> SAGSKSCDTVDLGYQCSPATSHLWGQYSPFFSLEDELSVSSKLPKDCRITLVQVLSRHGARYPTSSKSKKYKKLVTAIQANATDFKGKFAFLKTYNYTLGADDLTPFGEQQLVNSGIKFYQRYKALARSVVPFIRASGSDRVIASGEKFIEGFQQAKLADPGATNRAAPAISVIIPESETFNNTLDHGVCTKFEASQLGDEVAANFTALFAPDIRARAEKHLPGVTLTDEDVVSL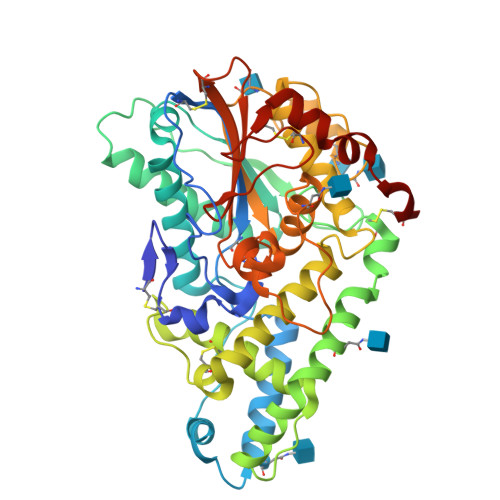MDMCSFDTVARTSDASQLSPFCQLFTHNEWKKYNYLQSLGKYYGYGAGNPLGPAQGIGFTNELIARLTRSPVQDHTSTNSTLVSNPATFPLNATMYVDFSHDNSMVSIFFALGLYNGTEPLSRTSVESAKELDGYSASWVVPFGARAYFETMQCKSEKEPLVRALINDRVVPLHGCDVDKLGRCKLNDFVKGLSWARSGGNWGECFS>MVWLANPERYGQMQYRYCGKSGLRLPALSLGLWHNFGHVNALESQRAILRKAFDLGITHFDLANNYGPPPGSAEENFGRLLREDFAAYRDELIISTKAGYDMWPGPYGSGGSRKYLLASLDQSLKRMGLEYVDIFYSHRVDENTPMEETASALAHAVQSGKALYVGISSYSPERTQKMVELLREWKIPLLIHQPSYNLLNRWVDKSGLLDTLQNNGVGCIAFTPLAQGLLTGKYLNGIPQDSRMHREGNKVRGLTPKMLTEANLNSLRLLNEMAQQRGQSMAQMALSWLLKDDRVTSVLIGASRAEQLEENVQALNNLTFSTKELAQIDQHIADGE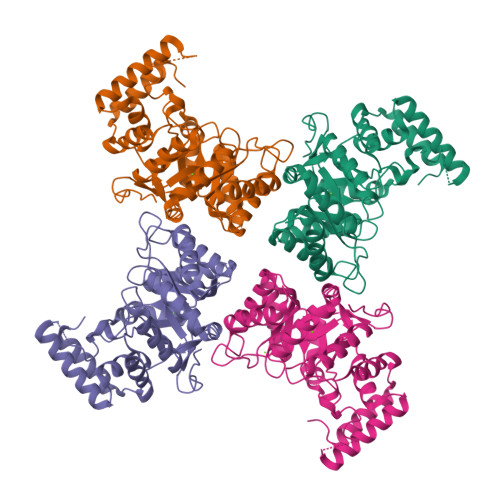LNLWQASSDK[8x]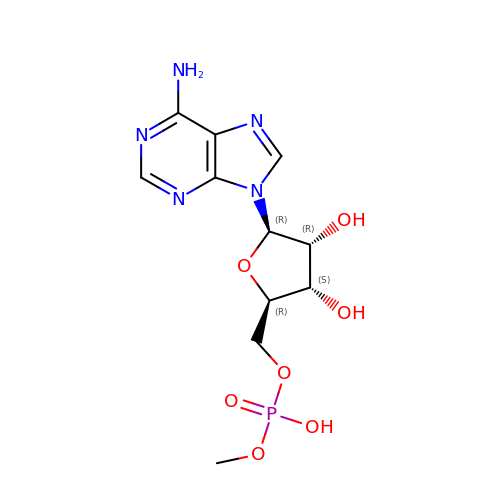5'-O-[(R)-hydroxy(methoxy)phosphoryl]adenosine | C11 H16 N5 O7 P | OYQVPLDFZZKUTQ-IOSLPCCCSA-N> MSVTVKRIIDNTVIVPKLPANEDPVEYPADYFRKSKEIPLYINTTKSLSDLRGYVYQGLKSGNVSIIHVNSYLYGALKDIRGKLDKDWSSFGINIGKAGDTIGIFDLVSLKALDGVLPDGVSDASRTSADDKWLPLYLLGLYRVGRTQMPEYRKKLMDGLTNQCKMINEQFEPLVPEGRDIFDVWGNDSNYTKIVAAVDMFFHMFKKHECASFRYGTIVSRFKDCAALATFGHLCKITGMSTEDVTTWILNREVADEMVQMMLPGQEIDKADSYMPYLIDFGLSSKSPYSSVKNPAFHFWGQLTALLLR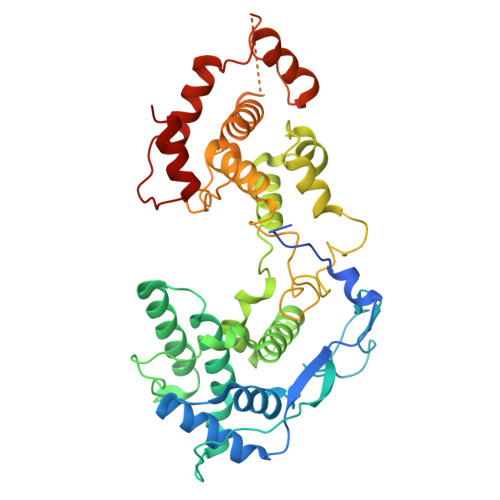STRARNARQPDDIEYTSLTTAGLLYAYAVGSSADLAQQFCVGDNKYTPDDSTGGLTTNAPPQGRDVVEWLGWFEDQNRKPTPDMMQYAKRAVMSLQGLREKTIGKYAKSEFDK9-[3-(4-fluorophenyl)-1-methyl-1H-pyrazol-4-yl]-2,3,4,5-tetrahydropyrido[2,3-f][1,4]oxazepine | C18 H17 F N4 O | 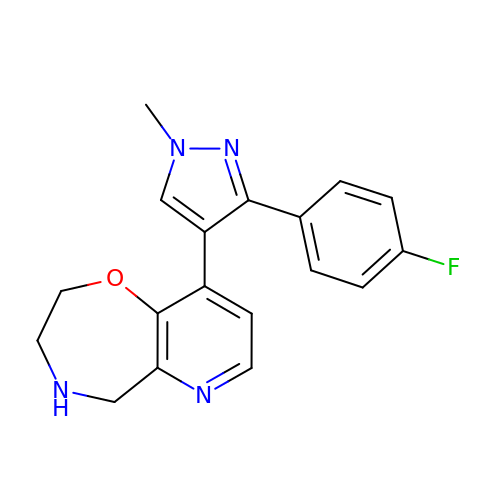RDUXJEGWTNOYDA-UHFFFAOYSA-N>MSKRFTTCATLISLVTAARAAYENAKQYEALCGAYAITKQAISDAEYIGDTTGDPRPKEVEDLYIMTLSDEDYNNKTLTGVTEEGGLEKRKSDILQRRDTYGREIHSIPANSEARAAAHVAIKRLFYKAGNLSANIAAAISSIKADTRSAGEALNRARCGQADCKAPDQKWFETRSKACSGTGEQKQGMTIASDISCLCSAATGETLCSAAATGGTYRGGEGTAANAQTDWSTTIADCDRNVEGKAPSPAAIEAAIAVFRAALGNAEFTKANSRKAFVLGHGSASDCNGGTSSAACVDYTNKLARGTINDIPWIEQLRTAAAKLAGVAGTRAQLDGMRQEMRIIEDQAWQAFALATIPLTAEKAKSQIVQQTKEED[6x]

Long-term immune evasion by the African trypanosome is achieved through repetitive cycles of surface protein replacement with antigenically distinct versions of the dense Variant Surface Glycoprotein (VSG) coat. The mature VSG proteins are attached to the cell surface by a GPI-anchor, and consist of two main regions: (1) a large, N-terminal domain (NTD) of roughly 300–400 amino acids that is most distal to the membrane and (2) a smaller, membrane-proximal C-terminal domain (CTD) spanning 80–120 amino acids beneath the NTD that harbors the GPI-anchor. Therefore, at the heart of antigenic variation in the African trypanosome are the NTDs of the VSGs. These large subdomains are elongated folds centered on a three-helix bundle scaffold.

VSG11 and VSG615 are related to VSG3 (the topologically-similar class of monomer/trimers with O-linked glycan PTMs), denoted as class B or N4 in the literature. NTD structures of VSG11 and VSG615 were solved to 1.23Å and 3.2Å resolution, respectively. Both reveal a fold similar to VSG3 as well as the presence of O-linked glycans on the top surface of the protein–one observed on VSG11 and two on VSG615. Interestingly, VSG615 crystallized with two trimers in the asymmetric unit, and these trimers align well with those of VSG3, VSG11, and VSG1954, providing additional support that class B trimer formation is not a crystallization artifact, but could represent the relevant, biological assembly. In contrast, in class B the bottom lobe residues are present at the N-terminal portion of the NTD sequence between the amino acids that form the first and second helices of the bundle. The second fact is that many of the class B VSGs are post-translationally modified by O-linked carbohydrates, whereas none of the class A VSGs have been found so modified. Finally, as noted in the Methods, the structures of VSG21, VSG545, VSG558, and VSG615 were solved by molecular replacement using an AlphaFold model of these VSGs as search models, indicating a very close fit of the model to the experimental data (a general idea for X-ray phasing implemented by several groups due to the accuracy of AlphaFold models).> GHMGRPRVARLDRERIAEAALELVDRDGDFRMPDLARHLNVQVSSIYHHAKGRAAVVELVRHRVVREIDGSAFERLPWDEAFSEWARSYRAAFS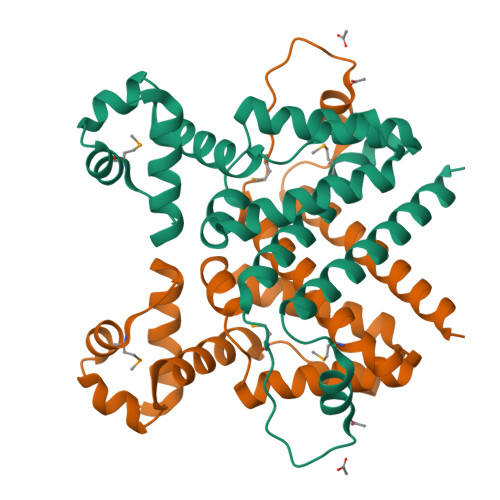RHPTAIRLLATETVRDPGSLSVYHSAAAGLRGAGFPDDHIMAVITAAENFLLGAALDAAAPEVMIEADSTTTDDALTRALAAAPRGPERAEQAFELGLAALLAGFHHLLQECGAVQRGS> MEVNPQFKKG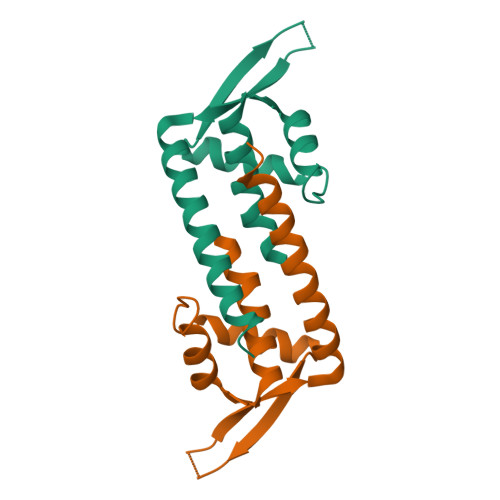VLELCCLFLIQKKDCYGYELANQVSKYIEVAEGAIYPVLRRLVKEEYCSTYLVESNEGPSRKYYQLTVKGEIYLNELISEWNNFTDSVAKLLTEGEAVNE> MGSDKIHHHHHHMIIAIPVSENRGKDSPISEHFGRAPYFAFVKVKNNAIADISVEENPLAQDHVHGAVPNFVKEKGAELVIVRGIGRRAIA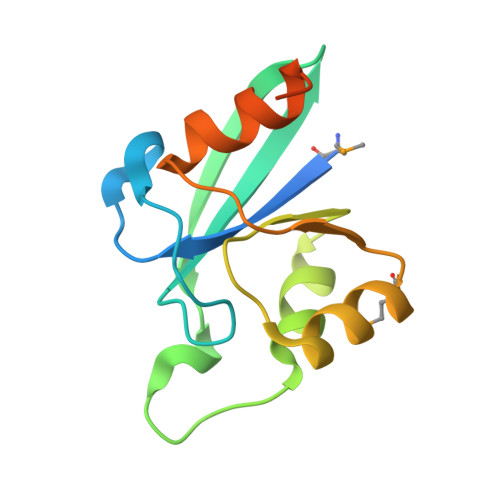AFEAMGVKVIKGASGTVEEVVNQYLSGQLKDSDYEVHDHHHHEHH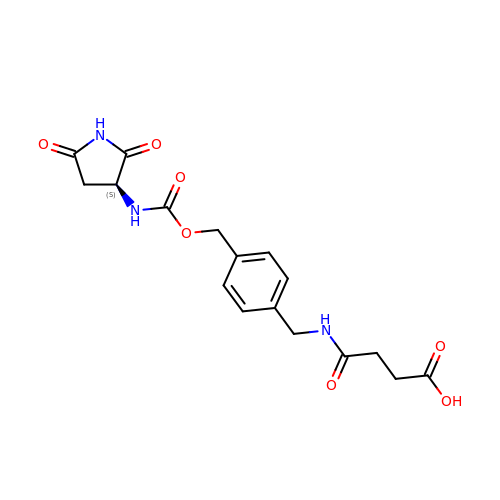4-[[4-[[(3~{S})-2,5-bis(oxidanylidene)pyrrolidin-3-yl]carbamoyloxymethyl]phenyl]methylamino]-4-oxidanylidene-butanoic acid | C17 H19 N3 O7 | GOZKVJYDZYJVDH-LBPRGKRZSA-N> MQIPASEQETLVRPKPLLLKLLKSVGAQKDTYTMKEVLFYLGQYIMTKRLYDEKQQHIVYCSNDLLGDLFGVPSFSVKEHRKIYTMIYRNLVVVN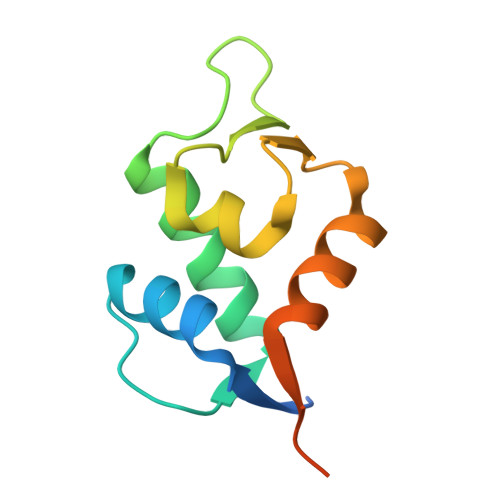QQESSDSGTSVSEN> MGSSHHHHHHSSGLVPRGSMSTSWSDRLQNAADMPANMDKHALKKYRREAYHRVFVNRSLAMEKIKCFGFDMDYTLAVYKSPEYESLGFELTVERLVSIGYPQELLSFAYDSTFPTRGLVFDTLYGNLLKVDAYGNLLVCAHGFNFIRGPETREQYPNKFIQRDDTE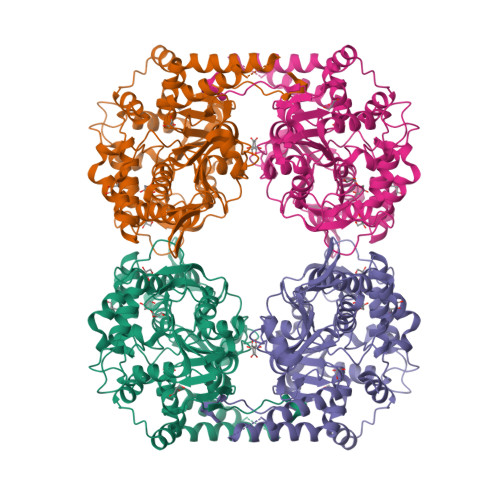RFYILNTLFNLPETYLLACLVDFFTNCPRYTSCETGFKDGDLFMSYRSMFQDVRDAVDWVHYKGSLKEKTVENLEKYVVKDGKLPLLLSRMKEVGKVFLATNSDYKYTDKIMTYLFDFPHGPKPGSSHRPWQSYFDLILVDARKPLFFGEGTVLRQVDTKTGKLKIGTYTGPLQHGIVYSGGSSDTICDLLGAKGKDILYIGDHIFGDILKSKKRQGWQTFLVIPELAQELHVWTDKSSLFEELQSLDIFLAELYKHLDSSSNERPDISSIQRRIKKVTHDMDMCYGMMGSLFRSGSRQTLFASQVMRYADLYAASFINLLYYPFSYLFRAAHVLMPHESTVEHTHVDINEMESPLATRNRTSVDFKDTDYKRHQLTRSISEIKPPNL>[4x]GKNGKGEVIIPKEKFWKISTPPEAYWNREQEK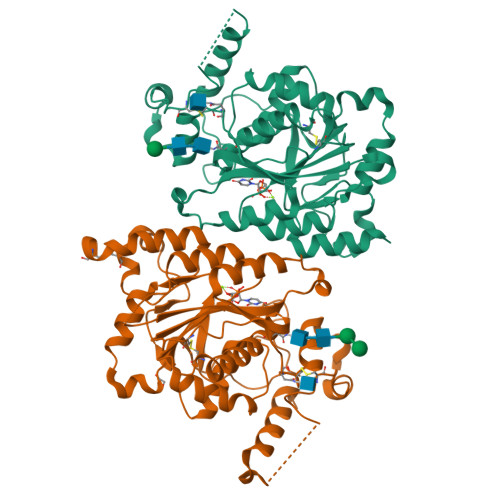LNRQYNPILSMLTNQTGEAGRLSNISHLNYCEPDLRVTSVVTGFNNLPDRFKDFLLYLRCRNYSLLIDQPDKCAKKPFLLLAIKSLTPHFARRQAIRESWGQESNAGNQTVVRVFLLGQTPPEDNHPDLSDMLKFESEKHQDILMWNYRDTFFNLSLKEVLFLRWVSTSCPDTEFVFKGDDDVFVNTHHILNYLNSLSKTKAKDLFIGDVIHNAGPHRDKKLKYYIPEVVYSGLYPPYAGGGGFLYSGHLALRLYHITDQVHLYPIDDVYTGMCLQKLGLVPEKHKGFRTFDIEEKNKNNICSYVDLMLVHSRKPQEMIDIWSQLQSAHLKC>[2x]MSTGTFVVSQPLNYRGGARVEPADASGTEKAFEPATGRVIATFTCSGEKEVNLAVQNAKAAFKIWSQKSGMERCRILLEAARIIREREDEIATMECINNGKSIFEARLDIDISWQCLEYYAGLAASMAGEHIQLPGGSFGYTRREPLGVCVGI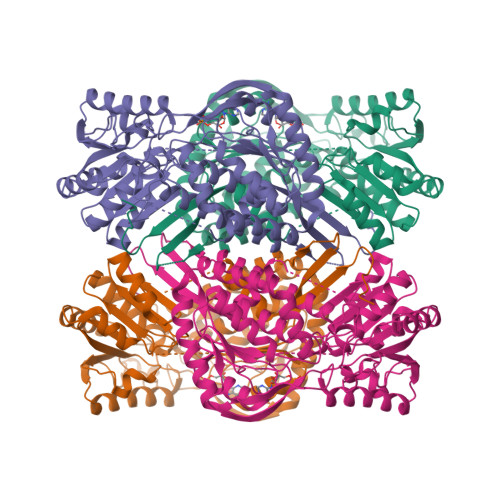GAWNYPFQIASWKSAPALACGNAMVFKPSPFTPVSALLLAEIYSEAGVPPGLFNVVQGGAATGQFLCQHPDVAKVSFTGSVPTGMKIMEMSAKGIKPVTLELGGKSPLIIFSDCDMNNAVKGALMANFLTQGQVCCNGTRVFVQKEILDKFTEEVVKQTQRIKIGDPLLEDTRMGPLINRPHLERVLGFVKVAKEQGAKVLCGGDIYVPEDPKLKDGYYMRPCVLTNCRDDMTCVKEEIFGPVMSILSFDTEAEVLERANDTTFGLAAGVFTRDIQRAHRVVAELQAGTCFINNYNVSPVELPFGGYKKSGFGRENGRVTIEYYSQLKTVCVEMGDVESAF>MVKEVVRTDSLKGRRGRLPSKPKSPQEPSPPSPPVSLISALVRAHVDSNPAMTSLDYSRFQANPDYQMSGDDTQHIQQFYDLLTGSMEIIRGWAEKIPGFADLPKADQD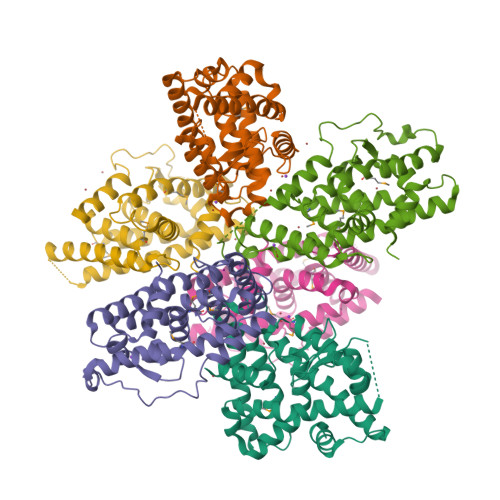LLFESAFLELFVLRLAYRSNPVEGKLIFCNGVVLHRLQCVRGFGEWIDSIVEFSSNLQNMNIDISAFSCIAALAMVTERHGLKEPKRVEELQNKIVNCLKDHVTFNNGGLNRPNYLSKLLGKLPELRTLCTQGLQRIFYLKLEDLVPPPAIIDKLFLDTLPF[6x]>DSCSEYCSNRCPSCDGQTQTQYTLCCINICCPS[3x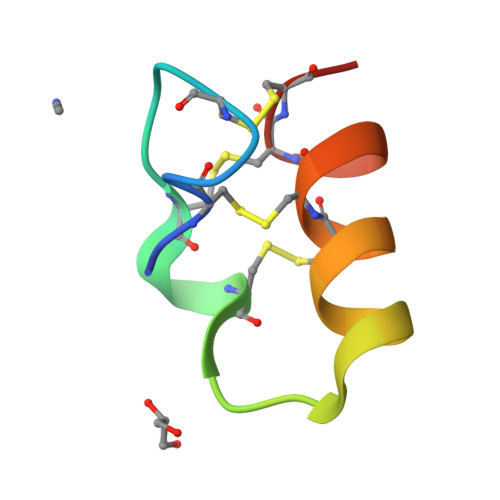]>SMADGNEDLRADDLPGPAFESYESMELACPAERSGHVAVSDGRHMFVWGGYKSNQVRGLYDFYLPREELWIYNMETGRWKKINTE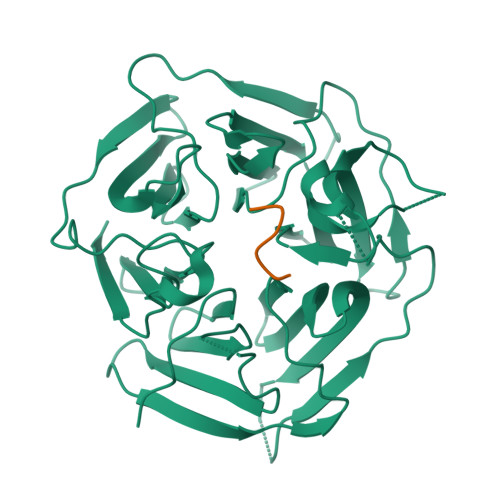GDVPPSMSGSCAVCVDRVLYLFGGHHSRGNTNKFYMLDSRSTDRVLQWERIDCQGIPPSSKDKLGVWVYKNKLIFFGGYGYLPEDKVLGTFEFDETSFWNSSHPRGWNDHVHILDTETFTWSQPITTGKAPSPRAAHACATVGNRGFVFGGRYRDARMNDLHYLNLDTWEWNELIPQGICPVGRSWHSLTPVSSDHLFLFGGFTTDKQPLSDAWTYCISKNEWIQFNHPYTEKPRLWHTACASDEGEVIVFGGCANNLLVHHRAAHSNEILIFSVQPK[2x];>GPSSGG[2x]>[2x]GAMIVKRLLGWKKG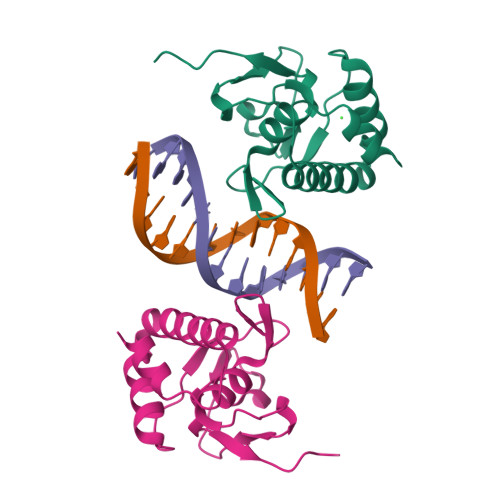EQNGQEEKWCEKAVKSLVKKLKKTGQLDELEKAITTQNVNTKCITIPRSLDGRLQVSHRKGLPHVIYCRLWRWPDLHSHHELRAMELCEFAFNMKKDEVCVNPYHYQRVETPVL3-ethyl-1-[(1~{R},8~{S},9~{S},10~{S})-10-oxidanyl-11-oxatricyclo[6.2.1.0^{2,7}]undeca-2(7),3,5-trien-9-yl]imidazolidine-2,4-dione | C15 H16 N2 O4 | 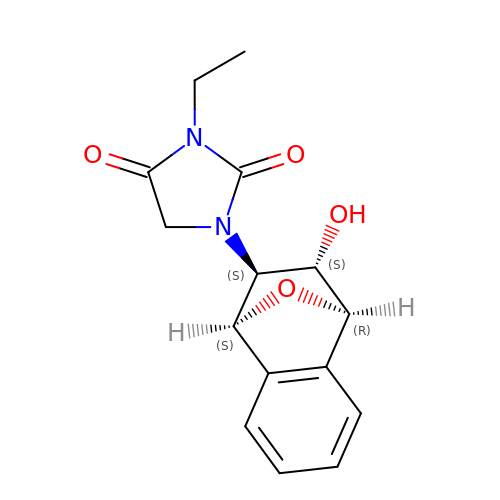GHZIAZMBFWRVPL-XDQVBPFNSA-N> GSSGSSGPGSLSGTEQAEMKMAVISEHLGLSWAELARELQFSVEDINRIRVENPNSLLEQSVALLNLWVIREGQNANMENLYTALQS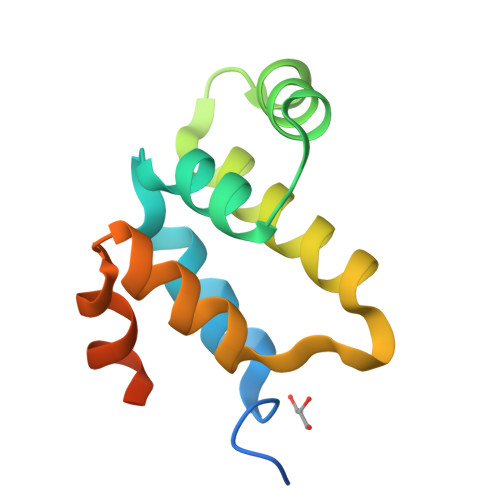IDRGEIVNMLEGSGRQSRNLKPDR> RALDRSIVKNLPEQFKNMYKYPSKMDNVLESWRTGLQSVDDAVMYM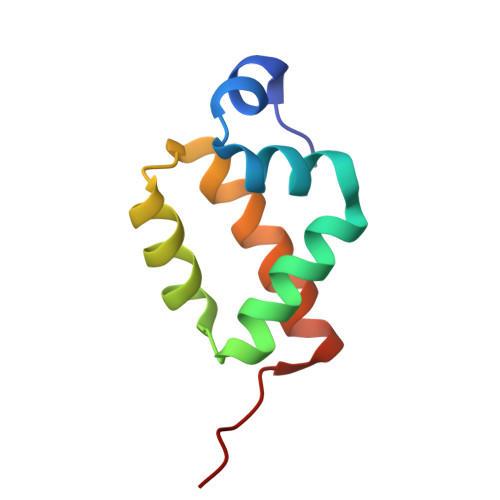KSLGMDFDAISHFVDAYRKHINKKGLPYAAA>MRGLSRRVQAMKPSATVAVNAKALELRRQGVDLVALTAGEPDFDTPEHVKEAARRALAQGKTKYAPPAGIPELREALAEKFRRENGLSVTPEETIVTVGGSQALFNLFQAILDPGDEVIVLSPYWVSYPEMVRFAGGVVVEVETLPEEGFVPDPERVRRAITPRTKALVVNSPNNPTGAVYPKEVLEALARLAVEHDFYLVSDEIYEHLLYEGEHFSPGRVAPEHTLTVNGAAKAFAMTGWRIGYACGPKEVIKAMASVSRQSTTSPDTIAQWA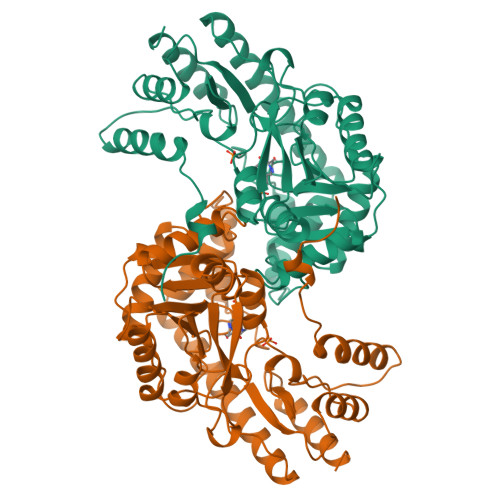TLEALTNQEASRAFVEMAREAYRRRRDLLLEGLTALGLKAVRPSGAFYVLMDTSPIAPDEVRAAERLLEAGVAVVPGTDFAAFGHVRLSYATSEENLRKALERFARVLGRA[2x]>SNAMNRLKNMSKYSDAKELASLTLGKKTEYANQYDPSLLQPVPRSLNRNDLHLSATLPFQGCDIWTLYELSWLNQKGLPQVAIGEVSIPATSANLIESKSFKLYLNSYNQTRFASWDEVQTRLVHDLSACAGETVTVNVKSLNEYTAEPIVTMQGECIDDQDIEIANYEFDDALLQGAAQGEEVSEVLHSHLLKS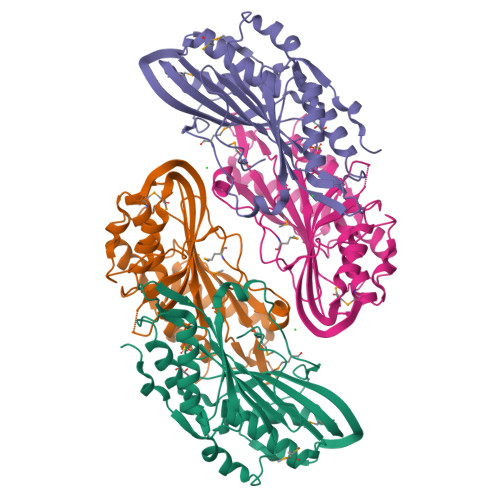NALITNQPDWGSVEIAYHGAKMNREALLRYLVSFREHNEFHEQCVERIFTDIMRYCQPQSLTVYARYTRRGGLDINPFRSSHQSAPNHNQRMARQ[2x]>[2x]HHHHHHMKEMSANTVLDSQRQQKHYGITSPISLASPKEIDHIYTQKLIDAMKPFGVFEDEEELNHRLVVLGKLNNLVKEWISDVSESKNLPPSVVATVGGKIFTFGSYRLGVHTKGADIDALCVAPRHVERSDFFQSFF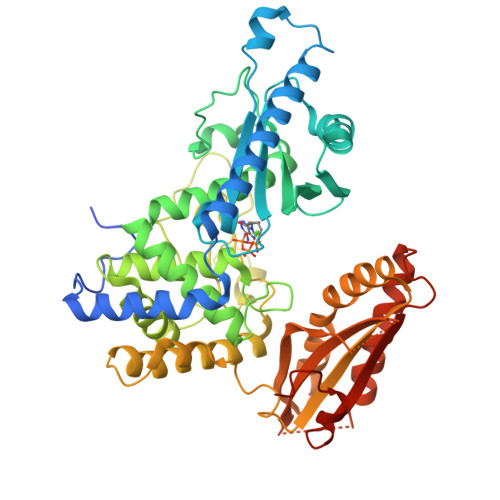EKLKHQDGIRNLRAVEDAFVPVIKFEFDGIEIDLVFARLAIQTISDNLDLRDDSRLRSLDIRCIRSLNGCRVTDEILHLVPNKETFRLTLRAVKLWAKRRGIYSNMLGFLGGVSWAMLVARTCQLYPNAAASTLVHKFFLVFSKWEWPNPVLLKQPEESNLNLPVWDPRVNPSDRYHLMPIITPAYPQQNSTYNVSTSTRTVMVEEFKQGLAVTDEILQGKSDWSKLLEPPNFFQKYRHYIVLTASASTEENHLEWVGLVESKIRVLVGNLERNEFITLAHVNPQSFPGNKEHHKDNNYVSMWFLGIIFRRVENAESVNIDLTYDIQSFTDTVYRQANNINMLKEGMKIEATHVKKKQLHHYLPAEILQKKKKQS>[6x]SNAMSELSYRRILLKLSGEALMGDGDYGIDPKVINRLAHEVIEAQQAGAQVALVIGGGN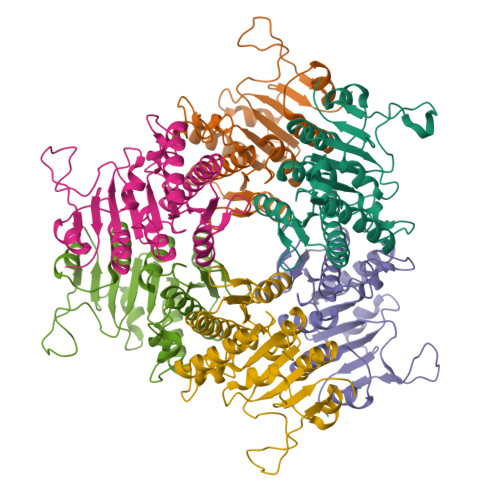IFRGAGLAASGMDRVTGDHMGMLATVINALAMQDALEKLGAKVRVMSAIKINDVCEDFIRRRAIRHLEKGRIAIFAAGTGNPFFTTDSGAALRAIEIGADLLLKATKVDGVYDKDPKKHSDAVRYDSLTYDEVIMQGLEVMDTAAFALARDSDLPLRIFGMSEPGVLLRILHGAQIGTLVQGRS> GPGGSMNSVFSGLDMLILLPYERRG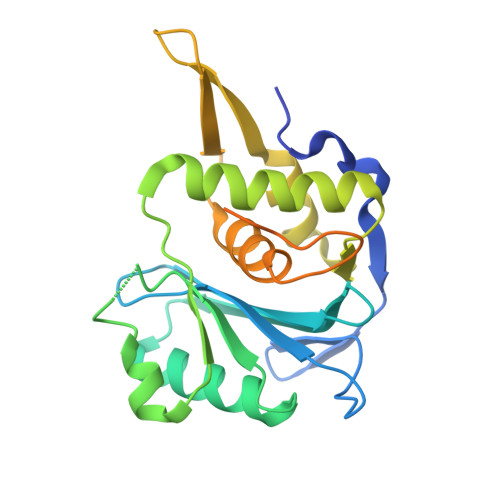TRLVVEDYRPDHIYCIGADFGKNQDYSVFSVLDLDTGAIVCLERMNGATWSDQVARLKALSEDYGHAYVVADTWGVGDAIAEELDAQGINYTPLPVKSSSVKEQLISNLALLMEKGQVAVPNDKTILDELRNFRYYRTASGNQVMRAYGRGHDDIVMSLALAYSQYEGKDGYKFELAEERPSKLKHEESVMSLVEDDFTDLELANRAFSAGLEHHHHHHHHHH> MQRSWFNHRLTSAKQKSLLYKSLADLVQSMMDTFVDPWLERITNRKSIFSMSKEDLETRTNELGQFFTIRTSNSSSVPMLLQQRLDEIHFKGTERPINQTIYREFNGISVLWDPIYAPVDLERHPYGTVLIPESTLETTGGTFGEMFLTSRGMIS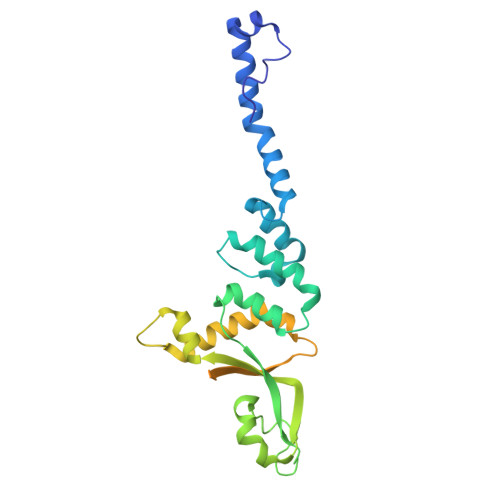IPINDLARTMGITGTIDQSAITEEILRKFNQFVKPLLPLHIVFDGLTLYLSVVVNEHADMITLNEISDTEKAYCWFETSDTTSLTGVTSISAPITATPGGTIVKATPTFDRTRADDLLLDSDA>[2x]GAPAITDPVKAGYDLAVRMDQVDTSQDSYSEAVMSINRGGKVLTRSFKTYSKHFGKDGKDEYSLI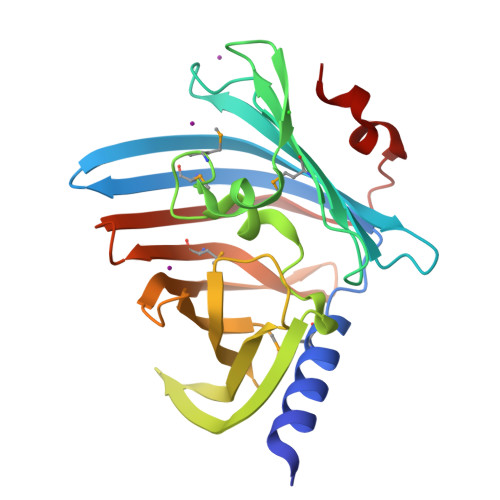VFDRPADVNGTKYLVWSYRGLEQDDDMWVYLPAESLVRRISGSSKFASFMRSDLSNEDIQNLDDVDEYDYLLQGEENVDGIDCYILERTPKKGKETQYSRQVQWVRKDTLLRLRADYYDKKDRLVKKLFFSRQEKIDGIWTVTQMRVERPREGSFTVIDWSNLRYDVGLSDAYFEHSALQR> MRIGIISVGPGNIMNLYRGVKRASENFEDVSIELVESPRNDLYDLLFIPGVGHFGEGMRRLRENDLIDFVRKHVEDERYVVGVCLGMQLLFEESEEAPGVKGLSLIEGNVVKLRSRRLPHMGWNEVIF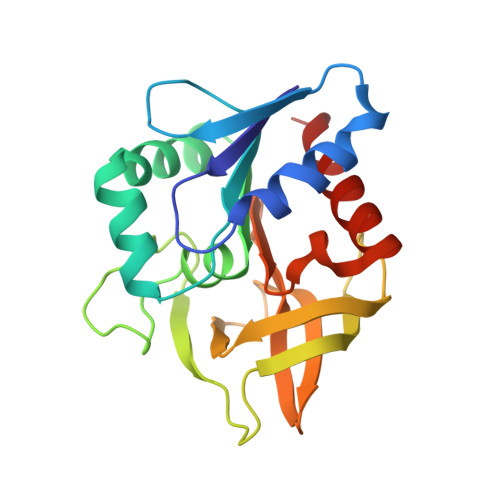KDTFPNGYYYFVHTYRAVCEEEHVLGTTEYDGEIFPSAVRKGRILGFQFHPEKSSKIGRKLLEKVIECSLSRR>MGGEVEEPEPQMVLSPLTSAAIFLVVTIDSGGEDTVRDLLSDVASLERAVGFRAQPDGRLSCVTGIGSEAWDRLFSGARPAGLHPFRELDGPVHRAVATPGDLLFHIRASRLDLCFALATEIMGRLRGAVTPQDEVHGFKYFDERDMLGFVAGTENPTGAAARRAVLVGAEDPAFAGGSYAVVQKYLHDIDAWEGLSVEAQERVIGRRKMTDVELSDDVKPADSHVALTSVTGPDGSDLEILRDNMPFGSVGREEFGTYFIGYARTPEVTETMLERMFLGTASAPHDRILDFSTAVTGSLFFTPAADFLEDLSARP[6x]

Using an X-ray free electron laser (XFEL), we have previously determined room-temperature (RT) serial femtosecond crystallography (SFX) structures of the ferric and Compound I redox states of DtpB,26 a B-type member of the dye-decolorizing peroxidase (DyP) family. Such an approach results in “pristine” DtpB structures that do not exhibit the effects of X-ray-generated radiation damage. The RT-SFX DtpB ferric and Compound I structures revealed that the distal heme pocket, which is composed of an Asp–Arg–Asn triad, was void of H2O molecules. DtpB, therefore, represents an exemplar of a His–heme-ligated peroxidase in which the distal heme pocket favors a dry site. By disrupting the distal heme pocket Asp–Asn–Arg triad in DtpB, our RT-SFX structures reveal that a wet site can be formed.

However, the lifetime (stability) of Compound I varies among the variants, with the D152A variant displaying no spectral changes for ∼1 h, while for the N245A and D152A/N245A variants, the Compound I spectrum decays toward that of an Fe(III)–heme spectrum within 10–15 min. Therefore, based on the D152A variant being the only variant having a Compound I species stable for >15 min, the ferric microcrystals of this variant were subjected to RT-SFX measurement following soaking with H2O2. Data collection and refinement statistics of the H2O2-soaked structure determined at 1.90 Å resolution are reported in Tables S1 and S2, respectively. The structure reveals that w2 and w3 remain present, with no new H2O molecule observed. An electron density peak is observed directly above the heme–Fe in each monomer of the hexamer assembly. However, owing to the longer Fe–O bond length, we are cautious to claim this structure as a “pure” Compound I species, where Fe–O bond lengths of between 1.63 and 1.73 Å are expected. The longer time scale for the extruder measurements may allow some decay of Compound I (see the kinetics of Compound I reduction below). A recent XFEL study reporting the Compound II structures of yeast cytochrome c peroxidase and ascorbate peroxidase highlights the possibility of flexibility inherent in Fe–O bond lengths between peroxidase species. However, regardless of whether an Fe(IV)=O or Fe(IV)–OH species is formed, Compound II bond lengths (1.76–1.88 Å)6,8,14,16,17,47,50−53 are consistently longer than Compound I bond lengths, and thus, for reasons further discussed below, it could be that the D152A H2O2-soaked structure is more representative of a Compound II species. A further point of note is that a wet site creates an additional H-bond donor to the oxo group.>[2x]MDMPVDPNEPT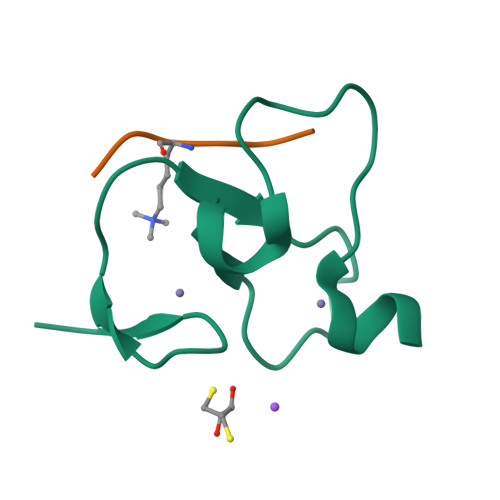YCLCHQVSYGEMIGCDNPDCSIEWFHFACVGLTTKPRGKWFCPRCSQER;>[2x]ARTKQTARKS>MKVPEAAISRLITYLRILEELEAQGVHRTSSEQLGELAQVTAFQVRKDLSYFGSYGTRGVGYTVPVLKRELRHILGLNRKWGLCIVGMGRLGSALADYPGFGESFELRGFFDVDPEKVGRPVRGGVIEHVDLLPQRVPGRIEIALLTVPREAAQKAADLLVAAGIKGILNFAPVVLEVPKEVAVE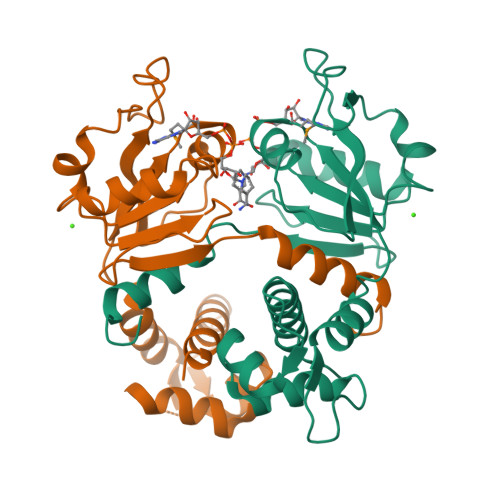NVDFLAGLTRLSFAILNPKWREEMMG[7x]> MADFARSLSITTPEEMIEKAKGETAYLPCKFTLSPEDQGPLDIEWLISPADNQKVDQVIILYSGDKIY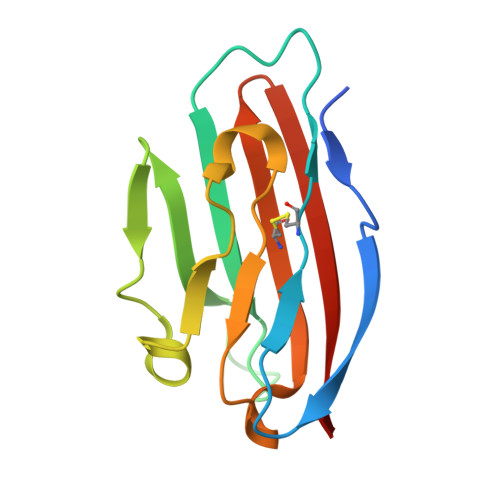DDYYPDLKGRVHFTSNDLKSGDASINVTNLQLSDIGTYQCKVKKAPGVANKKIHLVVLVK> SELYRQSLEIISRYLREQATGAKDTKPMGRSGA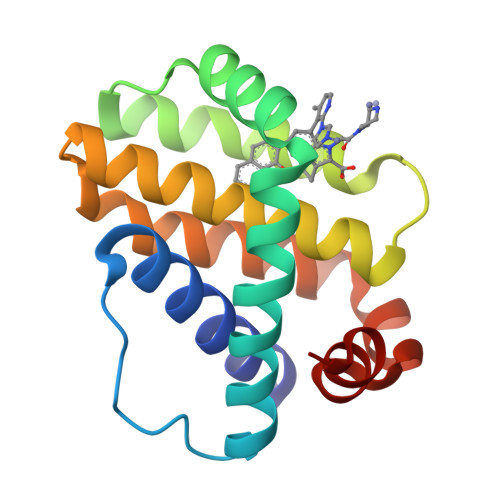TSRKALETLRRVGDGVQRNHETAFQGMLRKLDIKNEDDVKSLSRVMIHVFSDGVTNWGRIVTLISFGAFVAKHLKTINQESCIEPLAESITDVLVRTKRDWLVKQRGWDGFVEFFHV>[24x]MTSERTFIAVKPDGVQRCLVGEII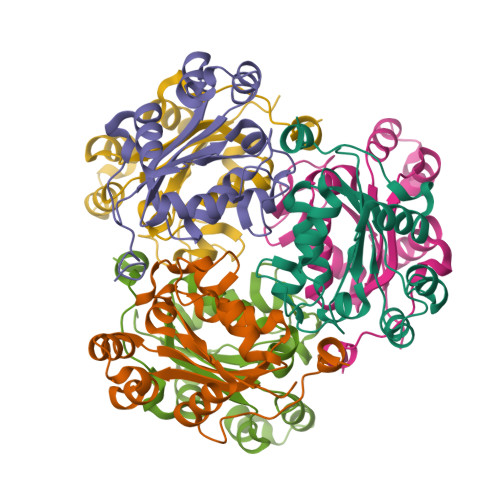QRFEKKGYKLVALKMLQPSAEQAQQHYIDLASKPFYKDLVAYFSSGPIVGMVWEGKGVVKGGRVLLGATNPADSLPGTIRGDFAVDVGRNVCHGSDSVDSAKREIAFWFKPEELVNWTSHSVKQVYE Ruminococcus bromii is a keystone species in the human gut that has the rare ability to degrade dietary resistant starch (RS). This bacterium secretes a suite of starch-active proteins that work together within larger complexes called amylosomes that allow R. bromii to bind and degrade RS. Starch adherence system protein 20 (Sas20) is one of the more abundant proteins assembled within amylosomes, but little could be predicted about its molecular features based on amino acid sequence. Here, we performed a structure–function analysis of Sas20 and determined that it features two discrete starch-binding domains separated by a flexible linker.

We solved the crystal structure of Sas20d1 via sulfur single-wavelength anomalous dispersion (SAD) phasing (2.1 Å, Rw = 17.7%, Rf = 21.4%) and then used this as a model to determine the structure with maltotriose (1.5 Å, Rw = 17.5%, Rf = 19.7%). The N-terminal β-sandwich most closely resembles a CBM26 module, which can be found adjacent to catalytic domains on α-amylases and typically binds maltoheptaose and β-cyclodextrin. A search on the DALI server showed that CBM26 from the Eubacterium rectale α-amylase Amy13K (ErCBM26) had the highest structural homology to Sas20d1 and aligns with an RMSD of ∼2.3 Å over 85 Cα atoms. While ErCBM26 and Sas20d1 share a conserved β-sandwich fold, two long loops formed by residues 146 to 161 (loop A) and 169 to 189 (loop B) protrude from Sas20d1 and are not found in ErCBM26. When comparing the native and maltotriose-bound Sas20d1 crystal structures, the CBM26-like fold at the N terminus is nearly identical. In the native structure, the α-helices at the C terminus of Sas20d1 are somewhat disordered with elevated B-factors compared with the rest of the structure, but in the maltotriose-bound structure, this region is well ordered. The Sas20d1 crystals with maltotriose (space group C2) have 45% solvent content and a tightly packed arrangement, with a crystal contact at the helical bundle. In each monomer, the helices (residues 237–257) are sandwiched between the same helical region (residues 237–257) and two β-strands (residues 58–70) of the neighboring monomer within the asymmetric unit and a loop (residues 93–104) of a symmetry-related monomer. This arrangement is in stark contrast to the native crystals, which were of the cubic space group I 21 3 and have ∼62% solvent. In these crystals, there are no crystal contacts in the region surrounding the helical bundle, which in part explains the elevated B-factors. Not surprisingly, the pocket of the native structure has an area of ∼783 Å2 and volume of ∼1350 Å3, whereas this space constricts to ∼521 Å2 and a volume of ∼848 Å3 in the maltotriose-bound structure.

> HHHHHHENLYFQGEETDTKIYFDASNLPAEWGTTKTVYCHLYAVAGDDLPETSWQGKAEKCKKDTATGLYYFDTAKLKSADGTNHGGLKDNADYAVIFSTIDTKSQSHQTCNVTLGKPCLGDTIYLTGGTVENTEDSSKRDFAATWKNNSDNYGPKAAITSLGHVTEGRFPIYLSRAEMVAQAIFNWAVKNPKNYTPETVADICAQVEAEPMDVYNAYAEMYATELADPAAYPDCAPLTTVATLLGVDPSG> SMNKKTKLIHGGHTTDDYTGAVTTPIYQTSTYLQDDIGDLRQGYEYSRTANPTRSSVESVIAALENGKHGFAFSSGVAAISAVVMLLDKGDHIILNSDVYGGTYRALTKVFTRFG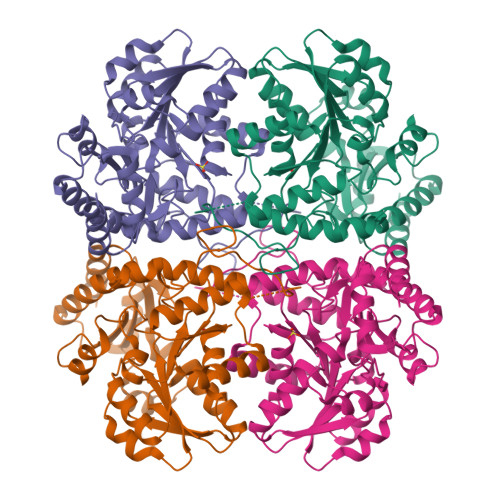IEVDFVDTTHTDSIVQAIRPTTKMLFIETPSNPLLRVTDIKKSAEIAKEHGLISVVDNTFMTPYYQNPLDLGIDIVLHSATKYLGGHSDVVAGLVATSDDKLAERLAFISNSTGGILGPQDSYLLVRGIKTLGLRMEQINRSVIEIIKMLQAHPAVQQVFHPSIESHLNHDVHMAQADGHTGVIAFEVKNTESAKQLIKATSYYTLAEALGAVESLISVPALMTHASIPADIRAKEGITDGLVRISVGIEDTEDLVDDLKQALDTL> GSMIFSVDKVRADFPVLSREVNGLPLAYLDSAASAQKPSQVIDAEAEFYRHGYAAVHRGIHTLSAQATEKMENVRKRASLFINARSAEELVFVRGTTEGINLVANSWGNSNVRAGDNIIISQMEHHANIVPWQMLCARVGAELRVIPLNPDGTLQLETLPTLFDEKTRLLAITHVSNVLGTENPLAEMITLAHQHGAKVLVDGAQAVMHHPVDVQALDCDFYVFSGHKLYGPTGIGILYVKEALLQEMPPWEGGGSMIATVSLSEGTTWTKAPWRFEAGTPNTGGIIGLGAALEYVSALGLNNIAEYEQNLMHYALSQLESVPDLTLYGPQNRLGVIAFNLGKHHAYDVGSFLDNYGIAVRTGHHCAMPLMAYYNVPAMCRASLAMYNTHEEVDRLV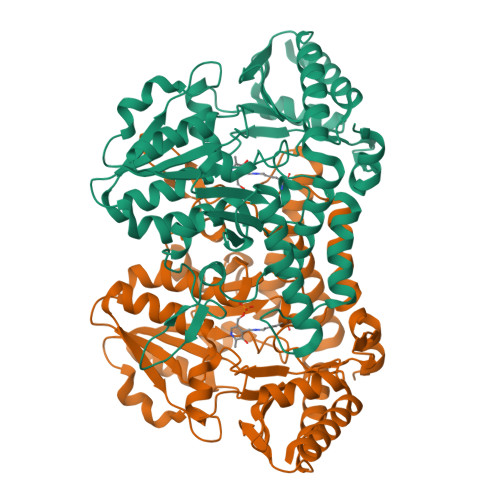TGLQRIHRLLG>[4x]GPGSMTGRVEGKVAFVTGAARGQGRSHAVRLAQEGADIIAVDICKPIRAGVVDTAIPASTPEDLAETADLVKGHNRRIVTAEVDVRDYDALKAAVDSGVEQLGRLDIIVANAGIG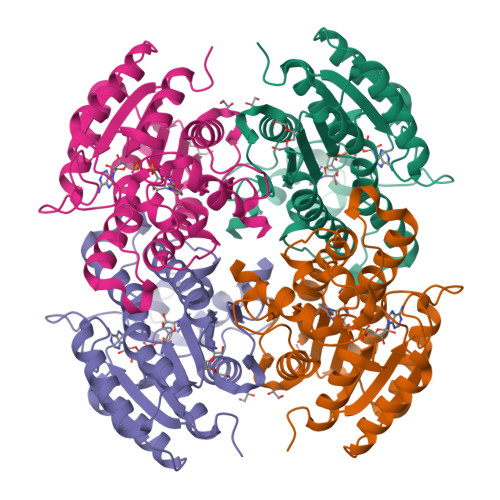NGGDTLDKTSEEDWTEMIDINLAGVWKTVKAGVPHMIAGGRGGSIILTSSVGGLKAYPHTGHYVAAKHGVVGLMRAFGVELGQHMIRVNSVHPTHVKTPMLHNEGTFKMFRPDLENPGPDDMAPICQMFHTLPIPWVEPIDISNAVLFFASDEARYITGVTLPIDAGSCLK>[2x]AEAGITGTWYNQLGSTF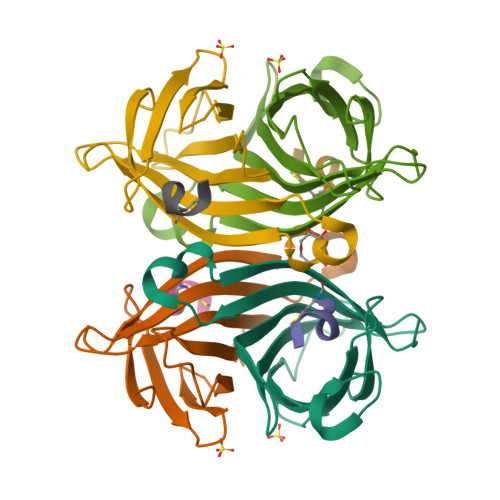IVTAGADGALTGTYESAVGNAESRYVLTGRYDSAPATDGSGTALGWTVAWKNNYRNAHSATTWSGQYVGGAEARINTQWLLTSGTTEANAWKSTLVGHDTFTKVKPSAAS;>MDVEAWL[2x]>[2x]MA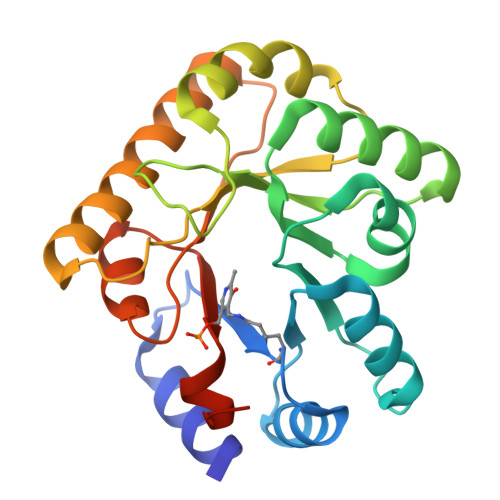QIAERLASLRSQLPPSVQLIAVSKNHPAAAIREAYAAGQRHFGENRVQEAIAKQAELTDLPDLTWHLLGKLQSNKARKAVEHFDWIHSVDSWALAERLDRIAGELGRSPKLCLQVKLLPDPNKAGWDPADLRAELPQLSQLQQVQIRGLMVIAPLGLTAAETQALFAQARTFAAELQQQAPQLRLTELSMGMSSDWPLAVAEGATWIRVGTQLFGPRSLEHHHHHH>SNAMDLSLLKALSEADAIASSEQEVRQILLEEAARLQKEVRFDGLGSVLIRLNESTGPKVMICAHMDEVGFMVRSISREGAIDVLPVGNVRMAARQLQPVRITTREECKIPGLLDGDRQGNDVSAMRVDIGARTYDEVMQAGIRPGDRVTFDTTF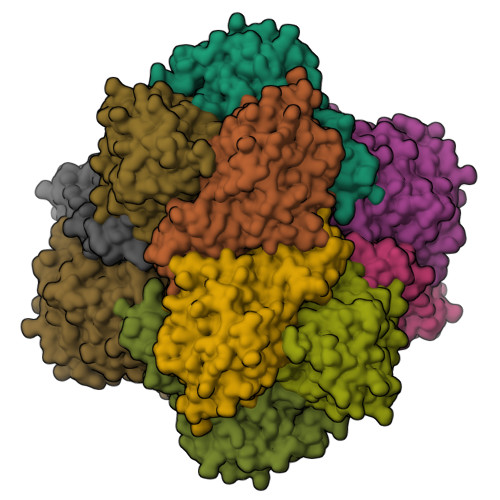QVLPHQRVMGKAFDDRLSCYLLVTLLRELHDAELPAEVWLVASSSEEVGLRGGQTATRAVSPDVAIVLDTACWAKNFDYGAANHRQIGNGPMLVLSDKSLIAPPKLTAWIETVAAEIGVPLQADMFSNGGTDGGAVHLTGTGVPTLVMGPATRHGHCAASIADCRDILQMEQLLSALIQRLTRETVVQLTDFR[6x]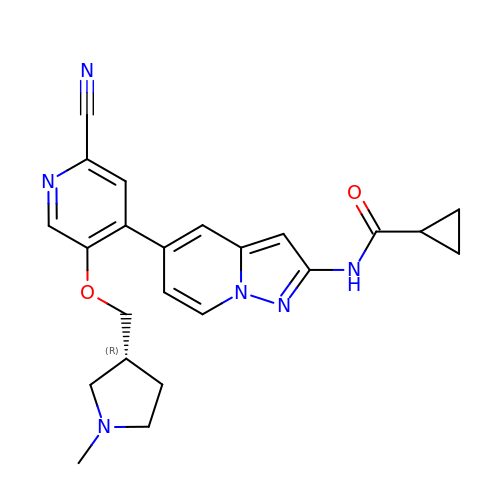N-[(5P,8R)-5-(2-cyano-5-{[(3R)-1-methylpyrrolidin-3-yl]methoxy}pyridin-4-yl)pyrazolo[1,5-a]pyridin-2-yl]cyclopropanecarboxamide | C23 H24 N6 O2 | GMHAIVQASIBHJM-OAHLLOKOSA-N>SNPYERGPDPTESSVTASRGPFATTTDSVSSLVSGFGGGTIYYPTDTSEGTFGGVVIAPGYTATQSSIAWMGHRIASQGFVVFTIDTNTRYDQPDSRGRQILAALDYLTQQSPVRDRVDPNRLAVMGHCMGGGGTLRAAENRPSLKAAIPLAPWHLQKDWSNVRVPTMIIGCENDTVASVSTHAIRFYESLPSSLPKAYLELRGADHFAPNRPNTTIAKYV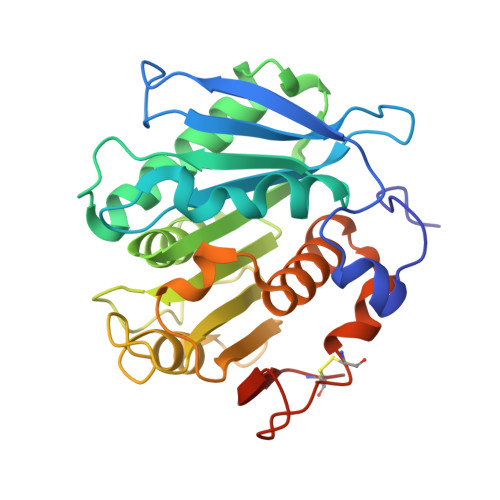IAWLKRFVDEDERYEQFLCPPPDTGLFSDFSDYRDSCPHTTLEHHHHHH[4x]2-[(8S)-4-oxo-2-(trifluoromethyl)-4,5-dihydropyrazolo[1,5-a]pyrazin-6-yl]acetamide | C9 H7 F3 N4 O2 | 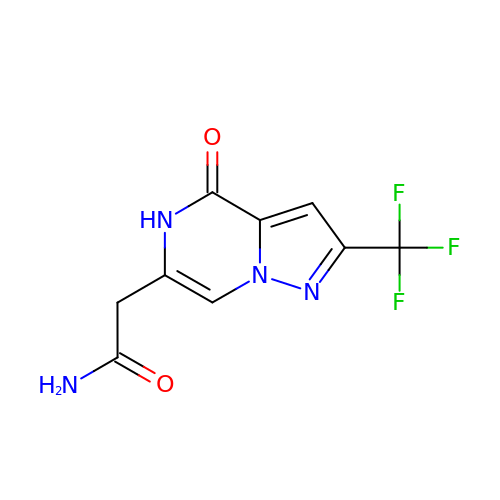NUSDSBLRWBKVLY-UHFFFAOYSA-N> DPSTYADYF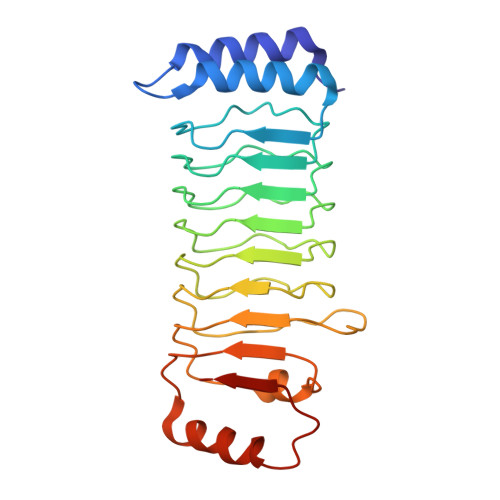SAWDKWEKQALPGEERDEAVSRLKECLINNSDELRLDRLNLSSLPDNLPAQITLLNVSYNQLTNLPELPVTLKKLYSASNKLSELPVLPPALESLQVQHNELENLPALPDSLLTMNISYNEIVSLPSLPQALKNLRATRNFLTELPAFSEGNNPVVREYFFDRNQISHIPESILNLRNECSIHISDNPLSSHALQALQRLTSSPDYHGPRIYFSMSD> AADFQGLYAEVKACSSELESLEMELRQQILVNIGKILQDQPSMEALEASLGQGLCSGGQVEPLDGPAGCILECLVLDSGELVPELAAPIFY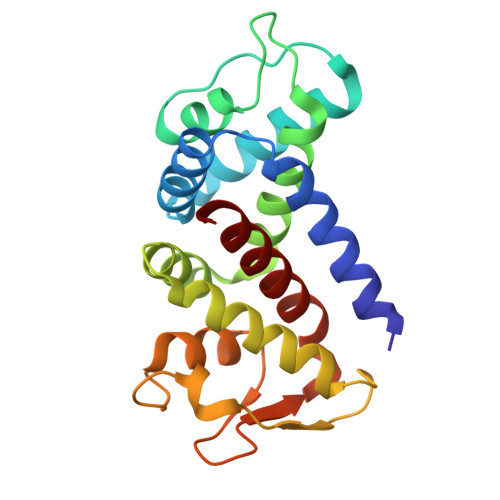LLGALAVLSETQQQLLAKALETTVLSKQLELVKHVLEQSTPWQEQSSVSLPTVLLGDCWDEKNPTWVLLEECGLRLQVESPQVHWEPTSLIPTSALYASLFLLSSLGQ>TPEKEPLKPGDILVYAQGGGEPKPIRLEELKPGDPFVLAYPMDPKTKVVKSGEAKNTLLVARFDPEELAPEVAQHAAEGVVAYSAVCTHLGCIVSQWVADEEAALCPCHGGVYDLRHGAQVIAGPPPRPVPQLPVR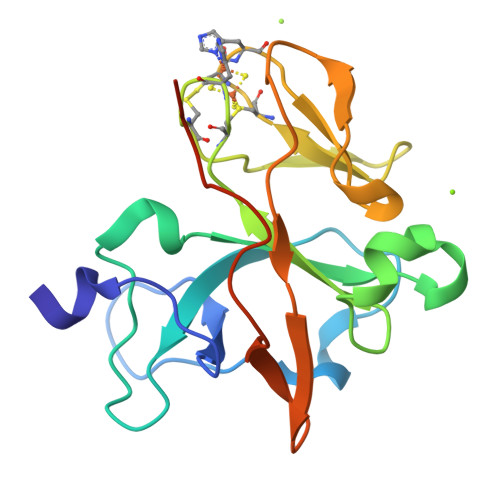VEDGVLVAAGEFLGPVGVQASAGAYTWRV[2x]>MKEVTIEIKNKTGLHARPAALFVQTASKFSSQIWVEKDNKKVNAKSIMGIMSLGVSQGNVVKLS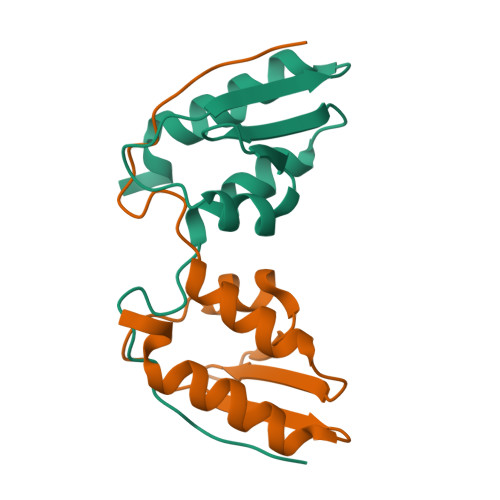AEGDDEEEAIKALVDLIESKFGEELEHHHHHH[2x]3-{5-[(2E,4aR,7aR)-6-(5-fluoro-4-methoxypyrimidin-2-yl)-2-imino-3-methyl-4-oxooctahydro-7aH-pyrrolo[3,4-d]pyrimidin-7a-yl]thiophen-3-yl}benzonitrile | C23 H20 F N7 O2 S | 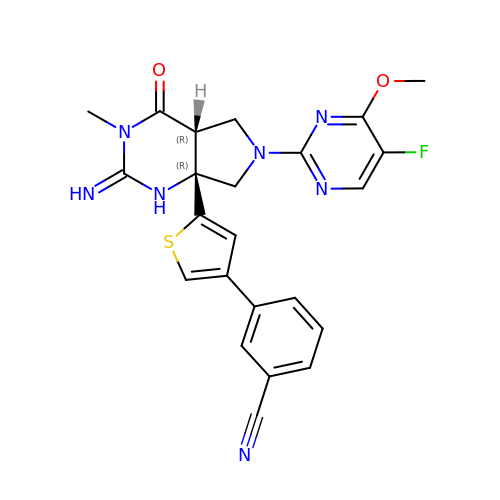UKGROMSNWKWCLS-HJPURHCSSA-N5-azanyl-3-[1-[[4-(pyrrolidin-1-ylmethyl)phenyl]methyl]indol-6-yl]-1~{H}-pyrazole-4-carbonitrile | C24 H24 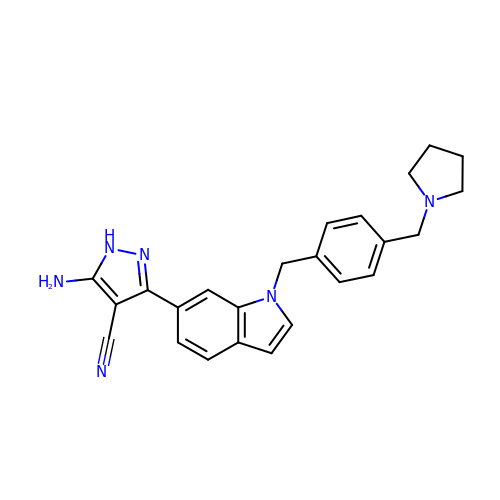N6 | IWWBYCSSMDZNIG-UHFFFAOYSA-N> A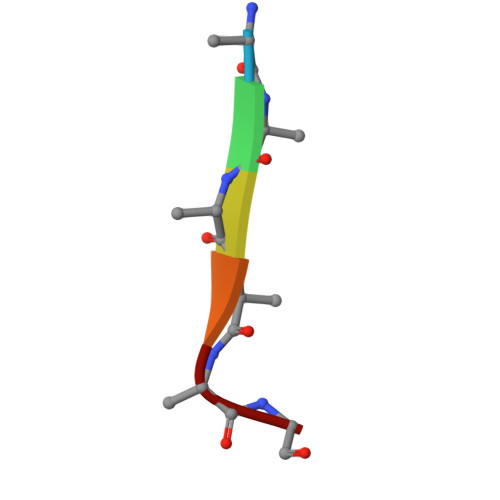AAAAG>GIDPFTMFRGVGTAIVTPFKNGELDLESYERLVRYQLENGVNALIVLGTTGESPTVNEDEREKLVSR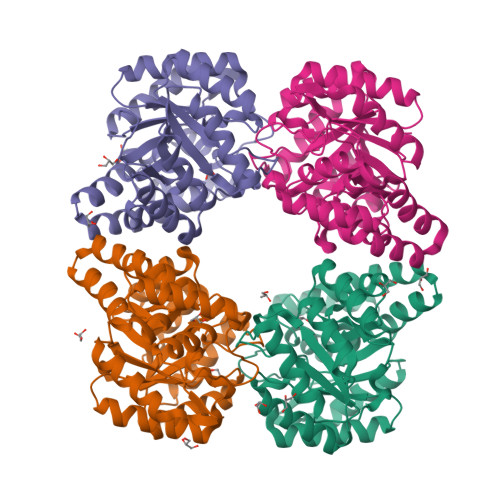TLEIVDGKIPVIVGAGTNSTEKTLKLVKQAEKLGANGVLVVTPYYNKPTQEGLYQHYKYISERTDLGIVVYNVPGRTGVNVLPETAARIAADLKNVVGIKEANPDIDQIDRTVSLTKQARSDFMVWSGNDDRTFYLLCAGGDGVISVVSNVAPKQMVELCAEYFSGNLEKSAEVHAKLRPLMKALFVETNPIPVKAALNLMGFIENELRLPLVPASEKTVELLRNVLKESGLL[6x]> MSAIFAERALLPEGWARNVRFEISADGVLAEIRPDANADGAERLGGAVLPGMPNLHSHAFQRAMAGLAEVAGNPNDSFWTWRELMYRMVARLSPEQIEVIACQLYIEMLKAGYTAVAEFHYVHHDLDGRSYADPAELSLRISRAASAAGIGLTLLPVLYSHAGFGGQPASEGQRRFINGSEAYLELLQRLRAPLEAAGHSLGLCFHS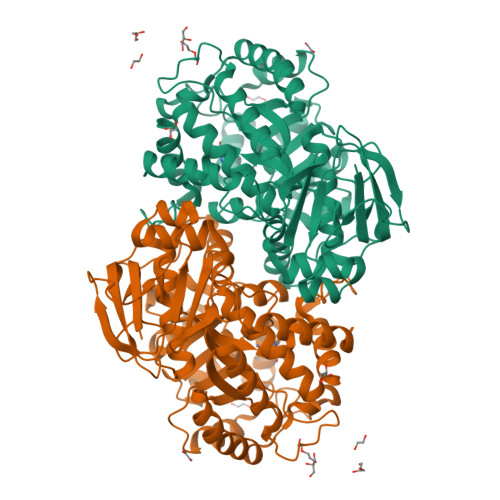LRAVTPQQIATVLAAGHDDLPVHIHIAEQQKEVDDCQAWSGRRPLQWLYENVAVDQRWCLVHATHADPAEVAAMARSGAVAGLCLSTEANLGDGIFPATDFLAQGGRLGIGSDSHVSLSVVEELRWLEYGQRLRDRKRNRLYRDDQPMIGRTLYDAALAGGAQALGQPIGSLAVGRRADLLVLDGNDPYLASAEGDALLNRWLFAGGDRQVRDVMVAGRWVVRDGRHAGEERSARAFVQVLGELLD>T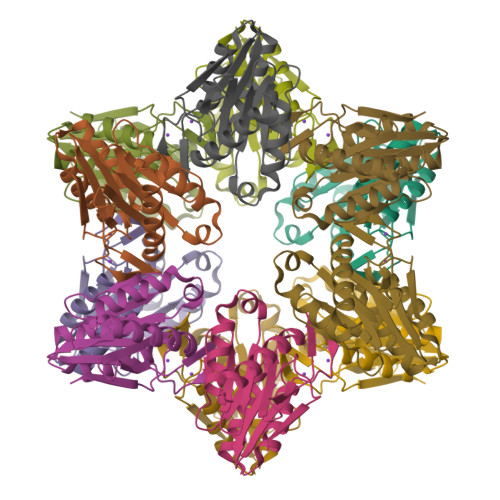TIVSVRRNGQVVVGGDGQVSLGNTVMKGNARKVRRLYNGKVLAGFAGGTADAFTLFELFERKLEMHQGHLLKSAVELAKDWRTDRALRKLEAMLIVADEKESLIITGIGDVVQPEEDQILAIGSGGNYALSAARALVENTELSAHEIVEKSLRIAGDICVFTNTNFTIEELPN[3x]> HHHHHHSSGLGVLFQGPGSKDFQGMLEYKRED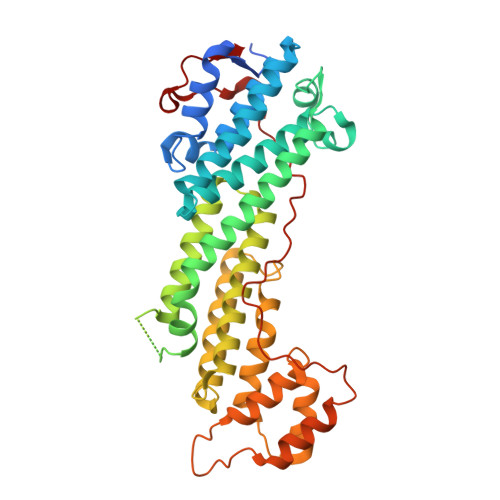EQKLVKNLILELKPRGVAVNLIPGLPAYILFMCVRHADYLNDDQKVRSLLTSTINSIKKVLKKRGDDFETVSFWLSNTCRFLHCLKQYSGEEGFMKHNTSRQNEHCLTNFDLAEYRQVLSDLAIQIYQQLVRVLENILQPMIVSGMLEHETIQGVSGVKPTGLRKRTSSIADEGTYTLDSILRQLNSFHSVMSQHGMDPELIKQVVKQMFYIVGAITLNNLLLRKDMCSWSKGMQIRYNVSQLEEWLRDKNLMNSGAKETLEPLIQAAQLLQVKKKTDDDAEAICSMCNALTTAQIVKVLNLYTPVNEFEERVSVSFIRTIQMRLRDRKDSPQLLMDAKHIFPVTFPFNPSSLALETIQIPASLGLGFIARV>MRGSHHHHHHGSWETEERPRTREEECHFYAGGQVYPGEASRVSVADHSLHLSKAKISKPAPYWEGTAVIDGEFKELKLTDYRGKYLVFFFYPLDFTFVCPTEIIAFGDRLEEFRSINTEVVACSVDSQFTHLAWINT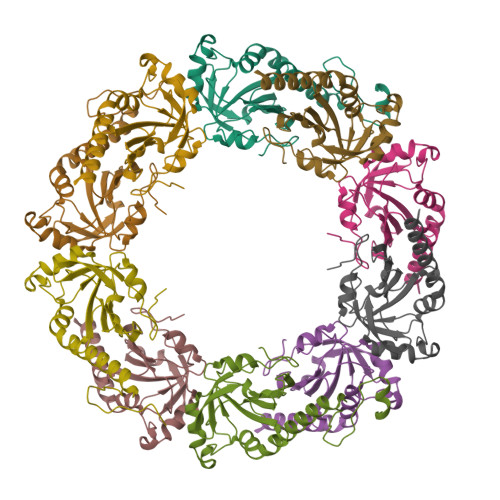PRRQGGLGPIRIPLLSDLTHQISKDYGVYLEDSGHTLRGLFIIDDKGILRQITLNDLPVGRSVDETLRLVQAFQYTDKHGEVCPAGWKPGSETIIPDPAGKLKYFDKLN[5x]The HpDnaB belongs to family 4 that consists of homohexameric replicative helicases. Each monomer consists of a N-terminal domain linked via a flexible linker to the C-terminal domain. Replicative helicases bind DnaG primase to synchronize DNA unwinding with RNA primer synthesis during the process of replication. To understand the roles played by NTD in helicase function, the importance of the linker region and helicase primase interactions, we present here the structure of NTD of HpDnaB at 2.2 Å resolution and compare it with other NTD structures.

We determined the structure of NTD of HpDnaB which is highly helical with a compact head (N-globe) and a long helix (H7) at the C-terminal end. The asymmetric unit consists of two complete monomers and two short peptide fragments. Interestingly, the two complete monomers form a dimer which is stabilized by the two short peptides and it eventually appears as a heterotetramer. In a dimer, the two monomers are arranged in a head-to-head manner where the C-terminal helices are extended parallel to each other. The two short peptides form helices, which are arranged in an anti-parallel fashion with the extended C-terminal helices (H7) resulting to the formation of a four helix bundle. The electron density suggested that these peptide sequences are similar to helix 7 and MALDI (Matrix-Assisted Laser Desorption/Ionization) analysis of crystals confirmed that these are degraded peptides of helix 7 from NTD itself. The dimeric interface consists of 29 hydrophobic residues that bury 3410.56 Å2 of solvent accessible surface area. The head-to-head dimer organization as seen in NTD of HpDnaB is different from other homologous structures known so far. However, the NTD of HpDnaB construct has a half of the helix hairpin (Helix 7) which does not allow the formation of four helix bundle as seen in the structure of MtbDnaB. Surprisingly, we observed that the NTD of HpDnaB shows very weak binding to HpDnaG primase compared to NTDL and HpDnaB, suggesting that N-terminal domain needs to be in a proper conformation for interaction with HpDnaG primase.

>[2x]MDHLKHLQQLQNIERIVLSGIVLANHKIEEVHSVLEPSDFYYPPNGLFFEIALKLHEEDCPIDENFIRQKMPKDKQIKEEDLVAIFAASPIDNIEAYVEEIKNASIKRKLFGLANTIREQAHH;> IKNASIKRKLFGLANTIREQAL;> VEEIKNASIKRKLFGLANTIREQALE>[2x]MASKVYDPEQRKRMITGPQWWARCAQMNVLDSFINYYDSEKHAENAVIFLHGNATSSYLWRHVVPHIEPVARCIIPDLIGMGKSGKSGNGSYRLLDHYKYLTAWFELLNLPKKIIFVGHDWGAALAFHYAYEHQDRIKAIVHMESVVDVIESWDE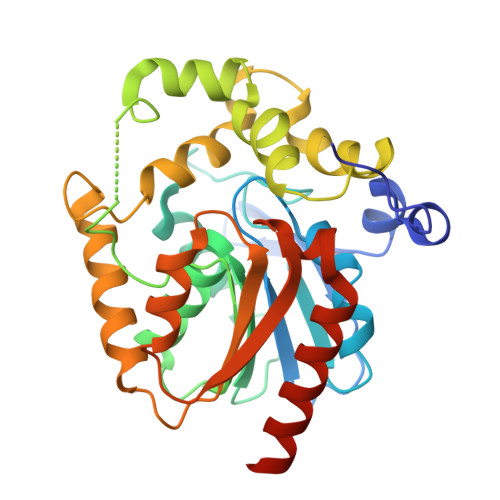WPDIEEDIALIKSEEGEKMVLENNFFVETVLPSKIMRKLEPEEFAAYLEPFKEKGEVRRPTLSWPREIPLVKGGKPDVVQIVRNYNAYLRASDDLPKLFIESDPGFFSNAIVEGAKKFPNTAFVKVKGLHFLQEDAPDEMGKYIKSFVERVLKNEQVDHHHHHH>VEKNITVTASVDPAIDLLQADGNALPSAVKLAYSPASKTFESYRVMTQVHTNDATKKVIVKLADTPQLTDVLNSTVQMPISVSWGG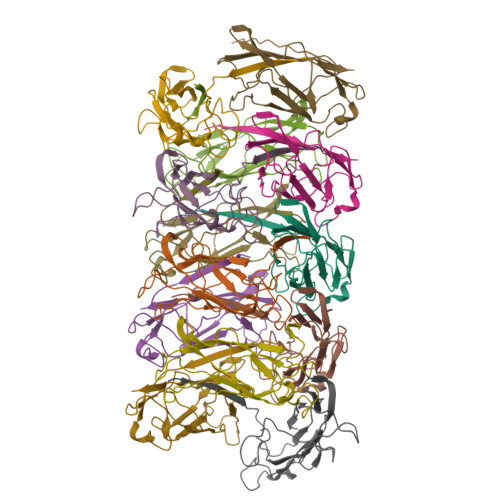QVLSTTAKEFEAAALGYSASGVNGVSSSQELVISAAPKTAGTAPTAGNYSGVVSLVMTLG[13x]>GSHMNINKQSPIPIYYQIMEQLKTQIKNGELQPDMPLPSEREYAEQFGISRMTVRQALSNLVNEGLLYRLKGRGTFVS[4x]

NagR, formerly termed YvoA, has been identified as a repressor protein from Bacillus subtilis that regulates genes involved in N-acetylglucosamine (GlcNAc) utilization. NagR acts as a negative transcriptional regulator, and binding of effector-free NagR to specific DNA operator sites blocks gene transcription. With more than 49000 deposited sequences, the GntR family of regulators (gluconate-operon repressor, Pfam family: PF00392) represents one of the largest groups of bacterial metabolite-responsive transcription factors. Their tertiary structure can be subdivided in almost all cases into two distinct domains: an N-terminal DNA-binding winged-helix-turn-helix (wHTH) domain and a C-terminal small-molecule effector-binding and oligomerization domain. In NagR and the entire GntR/HutC subfamily the C-terminal effector-binding domain adopts a so-called UTRA domain fold (Pfam family: PF07702) that is structurally homologous to the enzyme chorismate lyase.

In order to obtain more detailed insight into the DNA-binding determinants of NagR, we also solved the crystal structure of isolated NagR–DBDs in complex with an idealized 15mer palindromic operator dre-site at a resolution of 1.9 Å. Although the dsDNA fragment used for crystallization was designed to contain only a single palindromic dre-site, we observe not two but four NagR–DBD molecules bound to the dsDNA fragment in the structure of the complex. While two NagR–DBD molecules bind at the center of the dsDNA (as seen in the crystal structure of full-length NagR in complex with dsDNA), two additional NagR–DBDs bind at the edges of the dsDNA fragment. We propose that the two centrally bound NagR–DBDs show how NagR highly specifically recognizes DNA operator sites, while the two NagR–DBD molecules located at the edges of the dsDNA fragment reflect a considerably less specific interaction mode. The centrally bound NagR–DBDs interact closely with the sequence-specific recognition half-sites of the palindromic dsDNA with the sequence 5′-GTGGTCTAGACCAC-3′. While each NagR–DBD molecule contacts two contiguous segments of dsDNA, namely the nucleotides −7 to −4 from one strand and −3 to −1 from the opposite strand, sequence-specific interactions are restricted to the −7 to −4 segment and more precisely to bases G−7, G−5 and G−4. Thus, the wing motif reaches into the minor groove and contacts G−7 via the carbonyl oxygen of Gly69. The bases G−5 and G−4 are specifically recognized by Arg38 and Arg48, respectively. While Arg38 is located within the first helical turn of helix αD2, Arg48 extends from a similar position in helix αD3. Both arginine residues form bidental contacts with the guanine base they recognize, and the terminal side chain nitrogen atoms contact guanine atoms O6 or N7. The DBDs bound at the edges of the dsDNA fragment lack most base-specific interactions since only the wing anchoring via Gly69 is conserved.>[2x]MVLYFIGLGLYDERDIT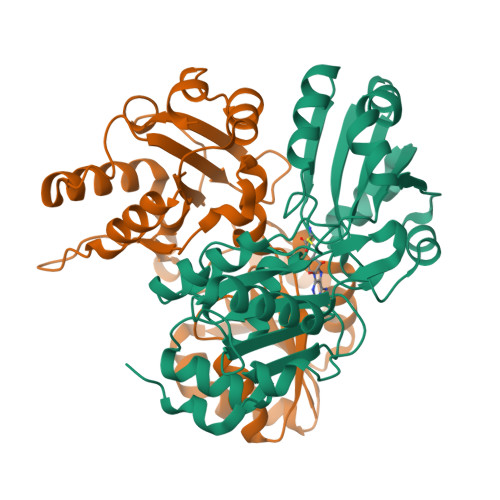VKGLEIAKKCDYVFAEFYTSLMAGTTLGRIQKLIGKEIRVLSREDVELNFENIVLPLAKENDVAFLTPGDPLVATTHAELRIRAKRAGVESYVIHAPSIYSAVGITGLHIYKFGKSATVAYPEGNWFPTSYYDVIKENAERGLHTLLFLDIKAEKRMYMTANEAMELLLKVEDMKKGGVFTDDTLVVVLARAGSLNPTIRAGYVKDLIREDFGDPPHILIVPGKLHIVEAEYLVEIAGAPREILRVNV2-[3-[3-[2,6-bis(azanyl)-5-(3-chlorophenyl)pyrimidin-4-yl]propoxy]phenoxy]ethanoic 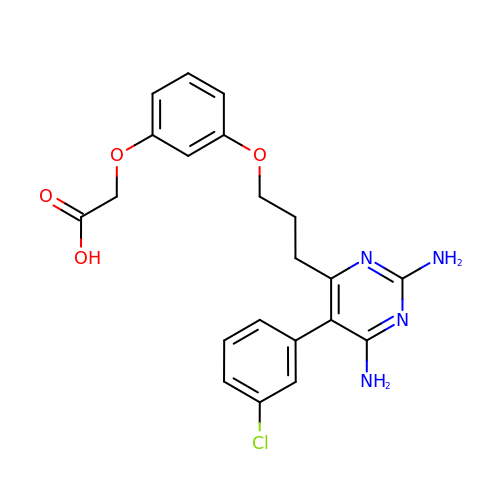acid | C21 H21 Cl N4 O4 | ABYWMEUIIHLYOL-UHFFFAOYSA-N>GPLGSSTMGQVGRQLAIIGDDINRRYDSEFQTMLQHLQPTAENAYEYFTKIATSLFESGINWGRVVALLGFGYRLALHVYQHGLT[2x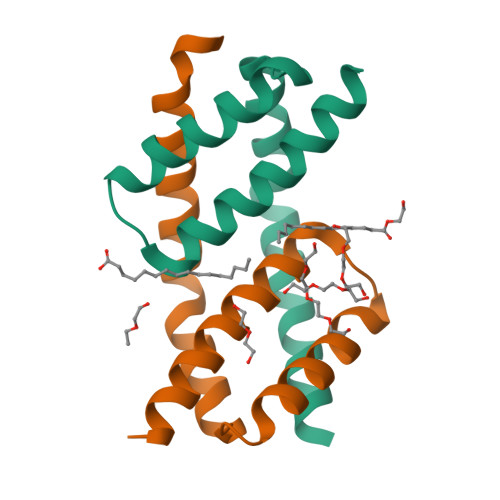]>LNSDGLTLLSLLKHLDRVPPQVTSTWKINASEATPCNWFGITCDDSKNVASLNFTRSRVSGQLGPEIGELKSLQILDLSTNNFSGTIPSTLGNCTKLATLDLSENGFSDKIPDTLDSLKRLEVLYLYINFLTGELPESLFRIPKLQVLYLDYNNLTGPIPQSIGDAKELVELSMYANQFSGNIPESIGNSSSLQILYLHRNKLVGSLPESLNLLGNLTTLFVGNNSLQGPVRFGSPNCKNLLTLDLSYNEFEGGVPPALGNCSSLDALVIVSGNLSGTIPSSLGMLKNLTILNLSENRLSGSIPAELGNCSSLNLLKLNDNQLVGGIPSALGKLRKLESL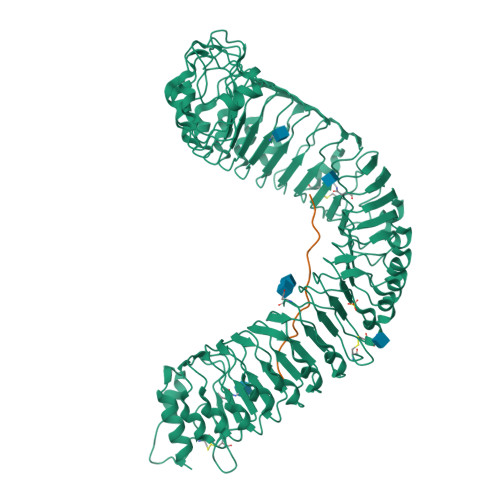ELFENRFSGEIPIEIWKSQSLTQLLVYQNNLTGELPVEMTEMKKLKIATLFNNSFYGAIPPGLGVNSSLEEVDFIGNKLTGEIPPNLCHGRKLRILNLGSNLLHGTIPASIGHCKTIRRFILRENNLSGLLPEFSQDHSLSFLDFNSNNFEGPIPGSLGSCKNLSSINLSRNRFTGQIPPQLGNLQNLGYMNLSRNLLEGSLPAQLSNCVSLERFDVGFNSLNGSVPSNFSNWKGLTTLVLSENRFSGGIPQFLPELKKLSTLQIARNAFGGEIPSSIGLIEDLIYDLDLSGNGLTGEIPAKLGDLIKLTRLNISNNNLTGSLSVLKGLTSLLHVDVSNNQFTGPIPDNLEGQLLSEPSSFSGNPNLCIP[2x];>KQRGKEKVSSGRPGQHN[2x]>[24x]SIPGQVADQAPLPSLAPMLEKVLPAVVSVRVEGTASQGQKIPEEFKKFFGDDLPDQPAQPFEGLGSGVIINASKGYVLTNNHVINQAQKISIQLNDGREFDAKLIGSDDQSDIALLQIQNPSKLTQIAIADSDKLRVGDFAVAVGNPFGLGQTATSGIVSALGRSGLNLEGLENFIQTDASINRGNAGGALLNLNGELIGINTAILA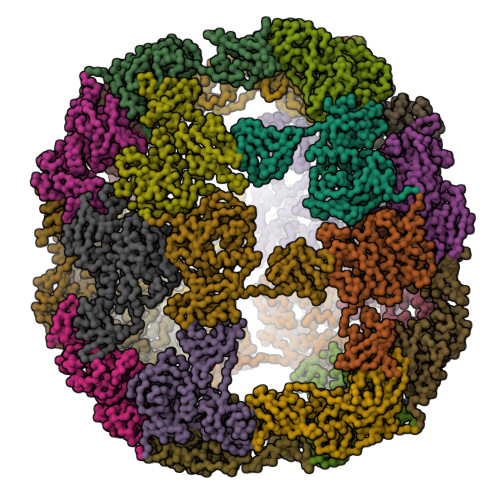PGGGSVGIGFAIPSNMARTLAQQLIDFGEIKRGLLGIKGTEMSADIAKAFNLDVQRGAFVSEVLPGSGSAKAGVKAGDIITSLNGKPLNSFAELRSRIATTEPGTKVKLGLLRNGKPLEVEVTLDTSTSSSASAEMITPALEGATLSDGQLKDGGKGIKIDEVVKGSPAAQAGLQKDDVIIGVNRDRVNSIAEMRKVLAAKPAIIALQIVRGNESIYLLMRLEHHHHHH> T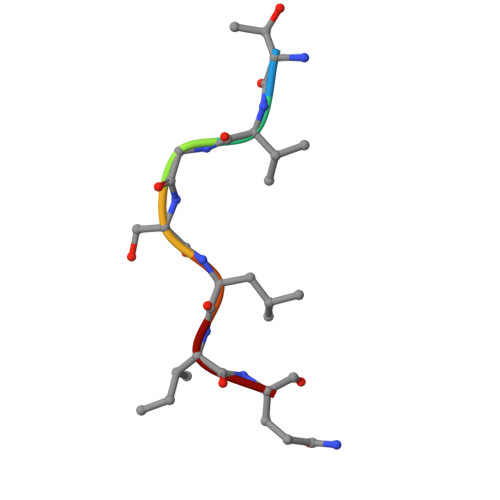VGSLIQ[3-(2-methoxy-2-oxidanylidene-ethoxy)phenyl]methyl 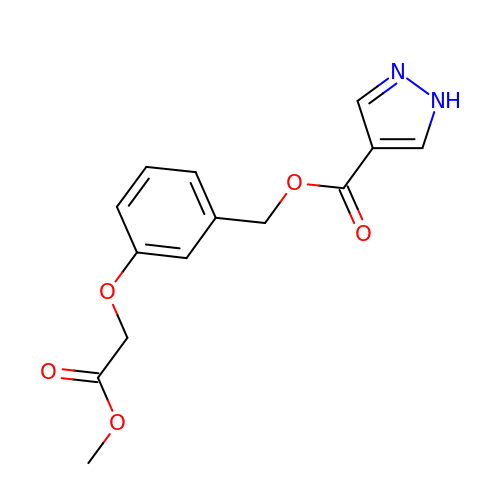1~{H}-pyrazole-4-carboxylate | C14 H14 N2 O5 | HARZTHMZNXIIKQ-UHFFFAOYSA-N> MTLSILVAHDLQRVIGFENQLPWHLPNDLKHVKKLSTGHTLVMGRKTFESIGKPLPNRRNVVLTSDTSFNV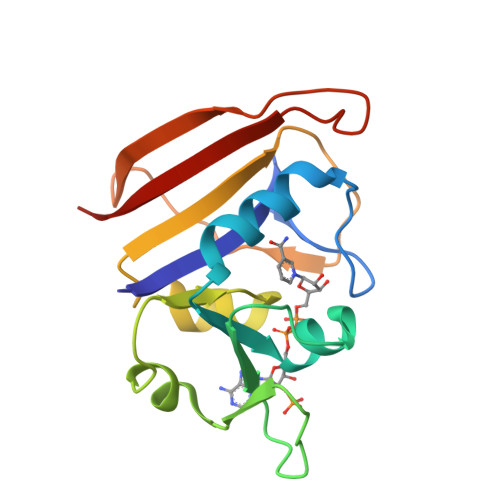EGVDVIHSIEDIYQLPGHVFIFGGQTLYEEMIDKVDDMYITVIEGKFRGDTFFPPYTFEDWEVASSVEGKLDEKNTIPHTFLHLIRKLE>[2x]MGSDKIHHHHHHMSNTVRAISPDITLFNKTLTFQEISQNTREAVIYIHGGAWNDPENTPNDFNQLANTIKSMDTESTVCQY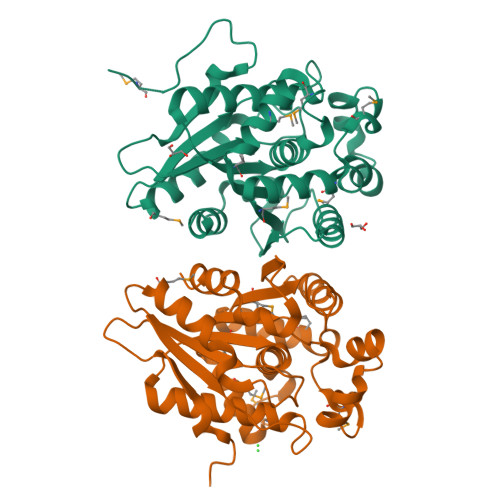SIEYRLSPEITNPRNLYDAVSNITRLVKEKGLTNINMVGHSVGATFIWQILAALKDPQEKMSEAQLQMLGLLQIVKRVFLLDGIYSLKELLIEYPEYDCFTRLAFPDGIQMYEEEPSRVMPYVKKALSRFSIDMHLVHSYSDELLTLRQTNCLISCLQDYQLSFKLYLDDLGLHNDVYKNGKVAKYIFDNIC> MSKIESALQAAQPGLSRLRGGAGGMGYRAATTQAEQPRSSLLDTIGRFAKAGADMYTAKEQRARDLADERSNEIIRKLTPEQRREALNNGTLLYQDDPYAMEALRVKTGRNAAYLVDDDVMQKIKEGVFRTREEMEEYRHSRLQEGAKVYAEQFGIDPEDVDYQRGFNGDITERNISLYGAHDNFLSQQAQKGAIMNSRVELNGVLQDPDMLRRPDSADFFEKYIDNGLVTGAIPSDAQATQLISQAFSDASSRAGGADFLMRVGDKKVTLNGATTTYRELIGEEQWNALMVTAQRSQFETDAKLNEQYRLKINSALNQEDPRTAWEMLQGIKAELDKVQPDEQMTPQREWLISAQEQVQNQMNAWTKAQAKALDDSMKSMNKLDVIDKQFQKRINGEWVSTDFKDMPVNENTGEFKHSDMVNYANKKLAEIDSMDIPDGAKDAMKLKYLQADSKDGAFRTAIGTMVTDAGQEWSAAVINGKLPERTPAMDALRRIRNADPQLIAALYPDQAELFLTMDMMDKQGIDPQVILDADRLTVKRSKEQRFEDDKAFESALNASKAPEIARMPASLRESARKIYDSVKYRSGNESMAMEQMTKFLKESTYTFTGDDVDGDTV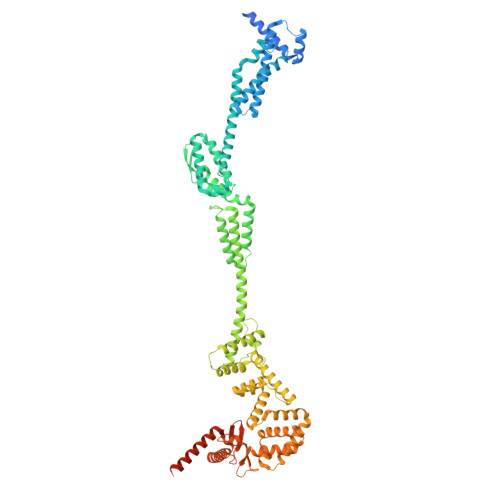GVIPKNMMQVNSDPKSWEQGRDILEEARKGIIASNPWITNKQLTMYSQGDSIYLMDTTGQVRVRYDKELLSKVWSENQKKLEEKAREKALADVNKRAPIVAATKAREAAAKRVREKRKQTPKFIYGRKE> MHSSLIILRHAYFSALHPARRVVPGSLLPVRTQFYTRHFTSTAGPTCGDGGETYKSEPTK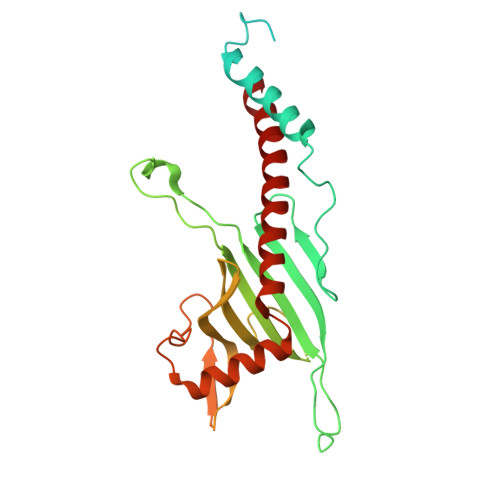VGASVEGTNSGNGVTDSPSLFSSSAPTVRRRALPPSDFPENALLKCIEKEIEDEALRLDKEECPPPPPTGWEMYHAPGTSVFYGRRWWLPATASAETRATPERHTIRVQLTKRDPSLDPECDVRGEHFPFSFFVQRAPSKGEAVRRDGTFRMGDSAAAGDVKGRTEGKEEEEEEEELGLYDQSIEVRADFVDGELLVDNVVFHGTFKTGSSCSKRSGNTSPEAAAATAAGQHDNTTGGRGKVEEVRYNNIFNGYPGPNLDEAEEEVLDGLQAWLAERCVDDQFGEFVGQYSVWVEQQEYEMWLKRLRDFVAA> DPTLEWFLSHCHIHKYPSKSTLIHQGEKAETLYYIVKGSVAVLIKDEEGKEMILSYLNQGDFIGELGLFEEGQERSA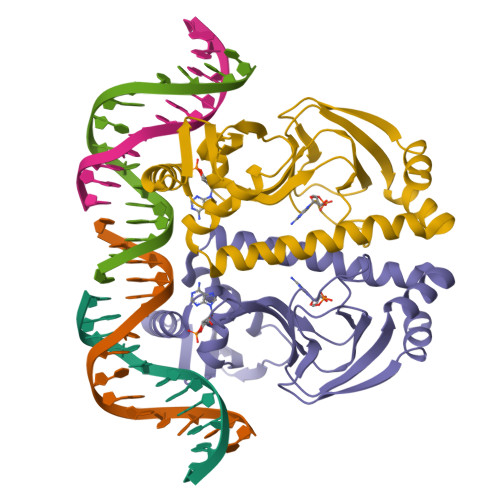WVRAKTACEVAEISYKKFRQLIQVNPDILMRLSAQMARRLQVTSEKVGNLAFLDVTGRIAQTLLNLAKQPDAMTHPDGMQIKITRQEIGQIVGCSRDTVGRILKMLEDQNLISAHGKTIVVYG> KDSLIMFLVEIFRSLFVSNCIDKNIDNVLLSIEEMFIDHYYNPQHSRLKYLIDDVGIFFTKLPITKAFHTYNKKYRITKRLYAPPTFNEVRHILNLAQILSLEEGLDLLTFDADETLYPDGHDFNDEVLASYISCLLKKMNIAIVTAASYNNDAEKYQKRLENLLKYFSKHNIKDGSYKNFYVMGGESNYLFKCNEEATLYSVPENEWRHYKKFVDYDTVQEILNISEKCLEKVIKDFGLCAQIQRKEKSIGLVPNKIPSLNIKNEQKNYMIKYEVLEEAVIRIKKEIIKNKITAPYCAFNGGQDLWVDVGNKAEGLLILQKLLKIQKKKCCHIGDQF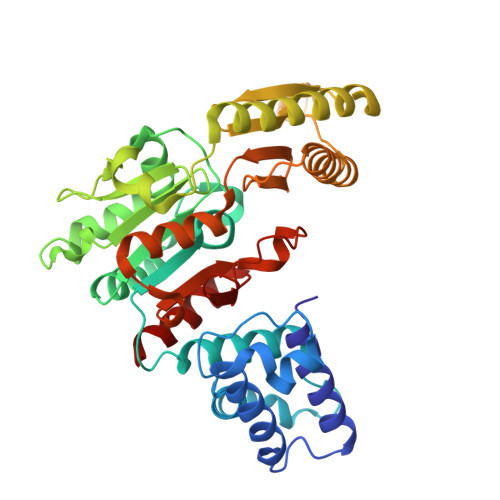LHSGNDFPTRFCSLTLWVSNPQETKACLKSIMHL>MAKVFQWFGSNESGAEFGSQNLPGVEGKDY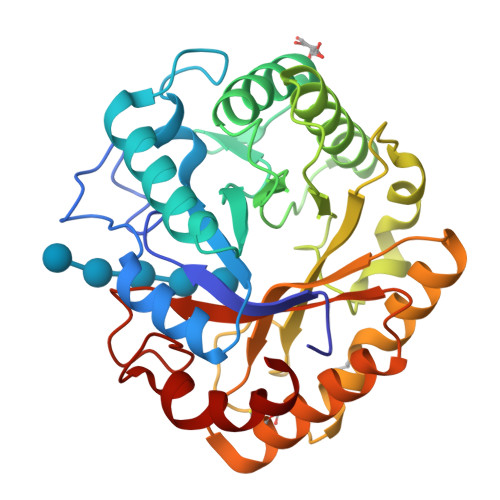IWPDPNTIDTLISKGMNIFRVPFMMERLVPNSMTGSPDPNYLADLIATVNAITQKGAYAVVDPHNYGRYYNSIISSPSDFQTFWKTVASQFASNPLVIFDTNNQYHDMDQTLVLNLNQAAIDGIRSAGATSQYIFVEGNSWTGAWTWTNVNDNMKSLTDPSDKIIYEMHQFLDSDGSGTSATCVSSTIGQERITSATQWLRANGKKGIIGEFAGGANDVCETAITGMLDYMAQNTDVWTGAIWWAAGPWWGDYIFSMEPDNGIAYQQILPILTPYL[2x]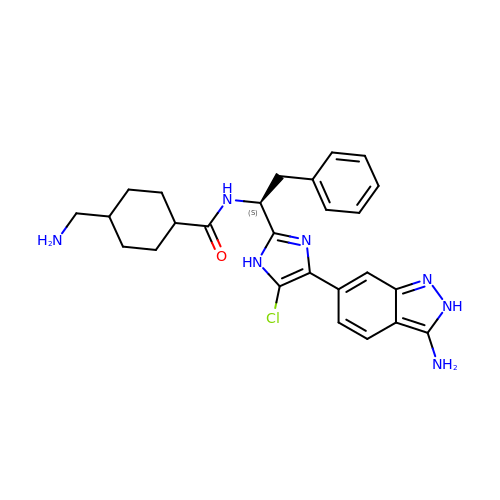trans-N-{(1S)-1-[4-(3-amino-2H-indazol-6-yl)-5-chloro-1H-imidazol-2-yl]-2-phenylethyl}-4-(aminomethyl)cyclohexane-1-carboxamide | C26 H30 Cl N7 O | IOLSRAXZCKDSPO-FIKGOQFSSA-N>MPFITVGQENSTSIDLYYEDHGTGTPVVLIHGFPLSGHSWERQSAALLDAGARVITYDRRGFGQSSQPTTGYDYDTFAADLNTVLETLDLQDAVLVGFSMGTGEVARYVSSYGTARIAAVAFLASLEPFLLKTDDNPDGAAPQEFFDGIVAAVKADRYAFYTGFFNDFYNLDENLGTRISEEAVRNSWNTAASGGFFAAAAAPTTWYTDFRADIPRIDVPALILHGTGDRTLPIENTARVFHKALPSAEYVEVEGAPHGLLWTHAEEVNTALLAFLAKAQEAQKQKLLTEVETYVLSIIPSGPLKAEIAQRLEDVFAGKNTDLEVLMEWLKTRPILSPLTKGILGFVFTLTVPSERGLQRRRFVQNALNGNGDPNNMDKAVKLYRKLKREITFHGAKEISLSYSAGALASCMGLIYNRMGAVTTEVAFGL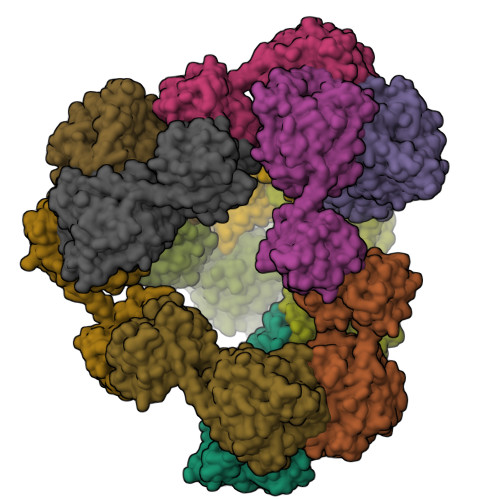VCATCEQIADSQHRSHRQLEHHHHHH[12x]> AS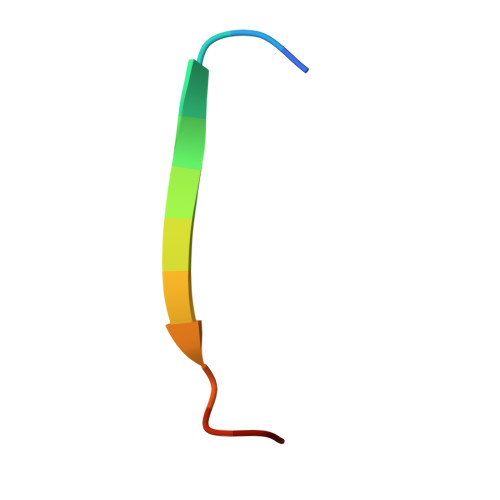GSSGTGSTGNQ> MAVPQFHRPSTVTTDSVRALGMRGLVLATNNSQFIMDNNHPHPQGTQGAVREFLRGQAAALTDLGLAHA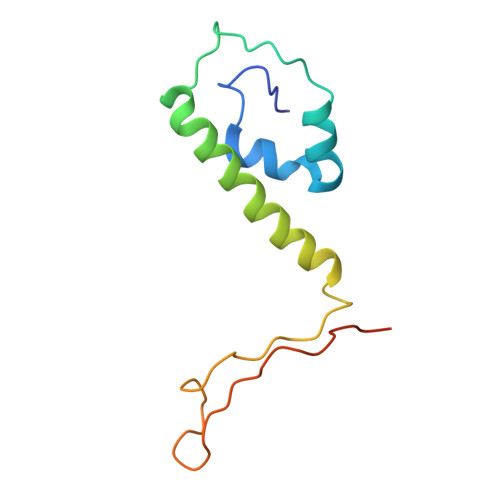NNTFTPQPMFAGDAPAAWLRPAFGLRRTYSPFVVREPSTPGTP>[3x]MKGTIVGTWIKTLRDLYGNDVVDESLKSVGWEPDRVITPLEDIDDDEVRRIFAKVSEKTGKNVNEIWREVGRQNIKTFSEWFPSYFAGR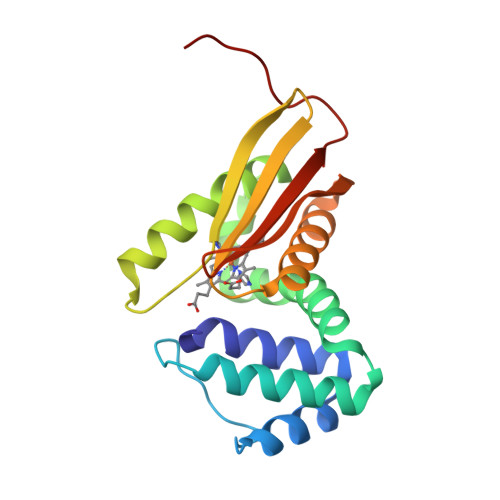RLVNFLMMMDEVGLQLTKMIKGATPPRLIAKPVAKDAIEMEYVSKRKMYDYFLGLIEGSSKFFKEEISVEEVERGEKDGFSRLKVRIKFKNPVFEYKKN>[2x]MAHHHHHHSSGLEVLFQGPAPKSGSTGKICKKTPEQLHMLKSAFVRTQWPSPEEYDKLAKESGLARTDIVSWFGDTRYAWKNGNLKWYYYYQSANS

Zhx1 to 3 (zinc-fingers and homeoboxes) form a set of paralogous genes encoding multi-domain proteins. ZHXs are multidomain proteins comprising two C2H2 zinc finger motifs and five homeodomains. In transient co-transfection assays ZHX isoforms have all been shown to function as transcriptional repressors. Whilst many 3-D structures of homeodomains have been determined by crystallography and NMR, we report two ZHX homeodomain structures which contain novel features.

Removal of the His tag was important for crystallizing ZHX1 HD4. Inspection of the crystal structure of ZHX1 HD4 (OPPF_2265) showed that, in addition to the normal homeodomain secondary structure, an extra helix is located at the C-terminal region. The additional C-terminal helix in HD4 we label as helix V in order to avoid confusion with an extension to helix III, present in certain homeodomains, referred to in earlier literature as helix IV. ZHX1 HD4 helix IV is fully ordered although no DNA is bound. Helix V in ZHX1 HD4 is positioned almost normal to both the plane of helices I & II as well as to helix III/IV, pointing away from the DNA major groove binding site on the latter. There is extensive interaction of hydrophobic side chains from helix V and particularly the C-terminal region of helix I. Many of the residues involved have aromatic side-chains including Tyr733, Trp732 and Tyr736. By contrast, for ZHX HD4 the network of ionic interactions is disrupted by the presence of apolar residues: Ala668 replacing Glu19 in engrailed whilst Met684 replaces Arg15. The fact that ZHX1 HD4 helix IV is ordered without the bound nucleic acid ligand could be a result of the presence of helix V where its interactions with helix I may help to anchor helix IV residues. Helix V is also unlikely to directly affect DNA binding as it points away from the expected major groove binding site. The two molecules in the asymmetric unit of ZHX1 HD4 crystal are related by pseudo translation, which was detected both by MOLREP and from a native self Patterson map.>[2x]GSHMKEDQVVAEEPGFQDEEESLF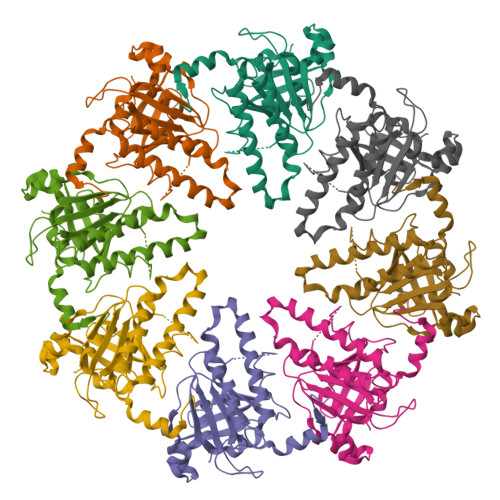QDIDLLQKHGINVADIKKLKSVGICTIKGIQMTTRRALCNVKGLSEAKVDKIKEAANKLIEPGFLTAFEYSEKRKMVFHITTGSQEFDKLLGGGIESMAITEAFGEFRTGKTQLSHTLCVTAQLPGAGGYPGGKIIFIDTENTFRPDRLRDIADRFNVDHDAVLDNVLYARAYTSEHQMELLDYVAAKFHEEAGIFKLLIIDSIMALFRVDFSGRGELAERQQKLAQMLSRLQKISEEYNVAVFVTNQMTADPGATMTFQADPKKPIGGHILAHASTTRISLRKGRGELRIAKIYDSPEMPENEATFAITAGGIGDAKE4-[3-(phenylsulfonylamino)prop-1-ynyl]benzenesulfonamide | C15 H14 N2 O4 S2 | 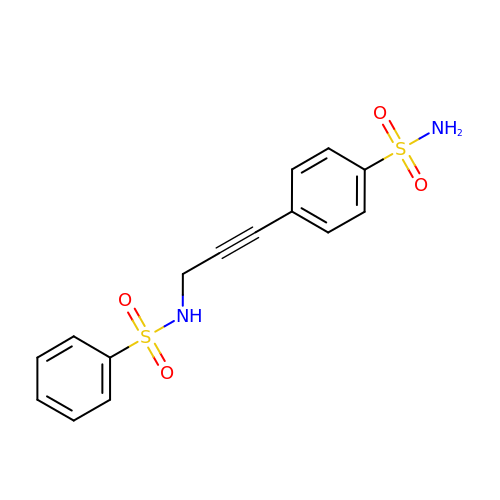CJZQAMWVHGWYBU-UHFFFAOYSA-N>[2x]ENEPKEGIPVDKKITVNKTWAVDGNEVNKADETVDAVFTLQVKQRYGEGTKKIEYDGQT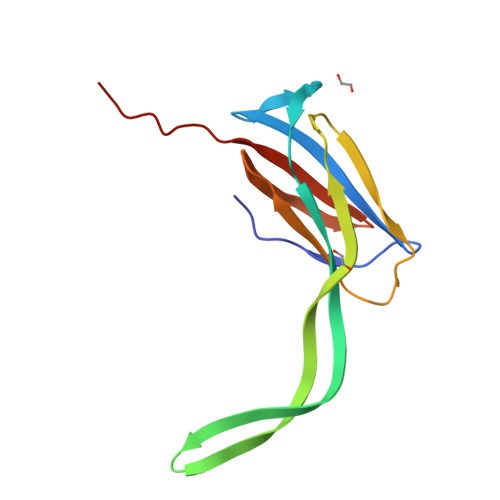YSIPSLFVKWVNVDSAKATAATSFKHTFENLDNAKTYRVIERVSGYAPEYVSFVNGVVTIKNNKDSNEPTPI> AKITFTNNCPNTVWPGTLTGDQKPQLSLTGFELASKASRSVDAPSPWSGRFWGRTRCSTDAAGKFT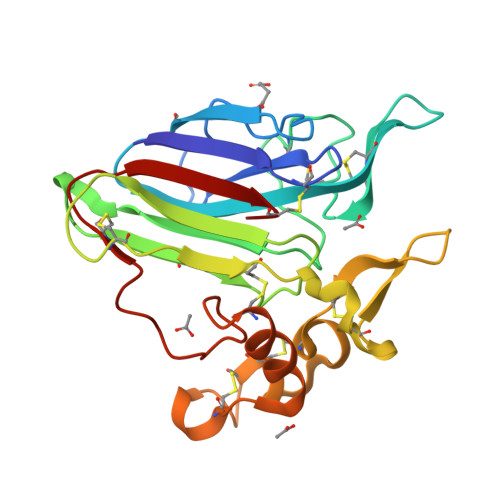CETADCGSGQVACNGAGAVPPATLVEITIAANGGQDYYDVSLVDGFNLPMSVAPQGGTGECKPSSCPANVNKVCPAPLQVKAADGSVISCKSACLAFGDSKYCCTPPNNTPETCPPTEYSEIFEKQCPQAYSYAYDDKNSTFTCSGGPDYVITFCP>GSENLYFQSGSMARQERAIRTRQTILVAAAEVFDEVGYEAATISDVLKRSGVTKGALYFHFTSKQELAQAVLAEQVASLPRVPEQELKLQQSLDEALLLAHLLREGTGDPIVQGSVRLTVDQGSPRDHLNRRVPMQAWTEHTQSLFEEARAKGEILPHADVEALAKLFVGAFTGVQVLSRIMTGR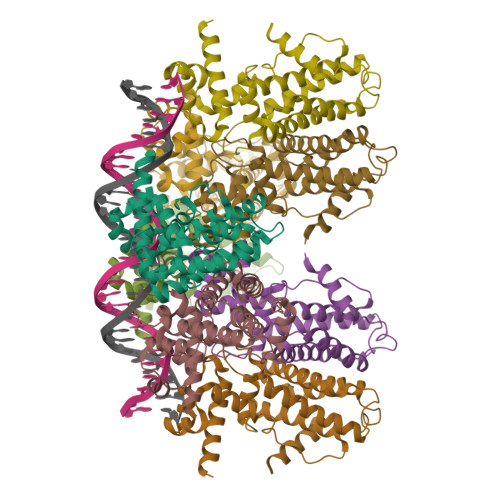ADLAERVADLYRHLMPSFAMPGILVRLDFSPERGSRVYEAAMKQRESAAASTTDAARTLE[8x]> EQAKAQLSNGYNNPNVNASNMYGPPQNMSLPPPQTQTIQGTDQPYQYSQCTGRRKALIIGINYIGSKNQLRGCINDAHNIFNFLTNGYGYSSDDIVILTDDQNDLVRVPTRANMIRAMQWLVKDAQPNDSLFLHYSGHGGQTEDLDGDEEDGMDDVIYPVDFETQGPIIDDEMHDIMVKPLQQGVRLTALFDSCHSGTVLDLPYTYSTKGI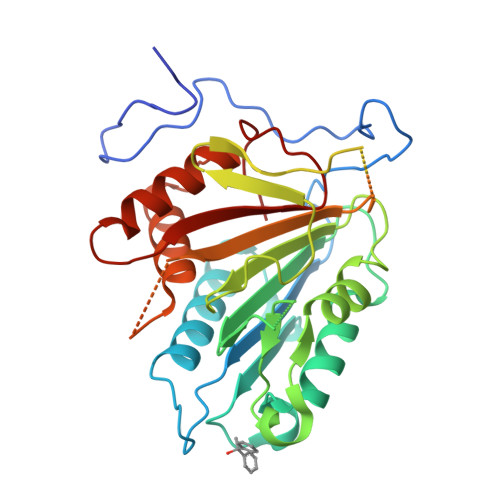IKEPNIWKDVGQDGLQAAISYATGNRAALIGSLGSIFKTVKGGMGNNVDRERVRQIKFSAADVVMLSGSKDNQTSADAVEDGQNTGAMSHAFIKVMTLQPQQSYLSLLQNMRKELAGKYSQKPQLSSSHPIDVNLQFIM> M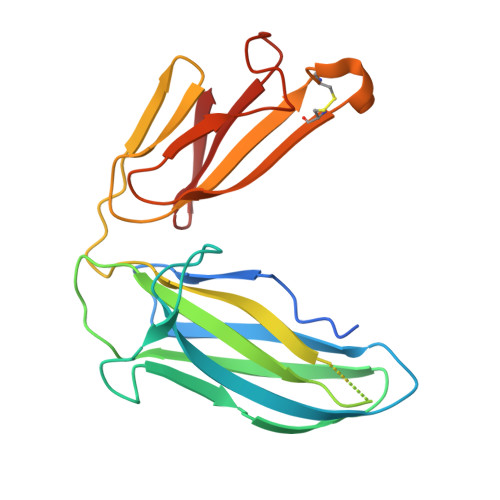AHHHHHHVDDDDKMLDVGDISSFMNSDSSTLSKTIQNSTDSGRLINIRLERLSSPLDDGQVIAMDKPDELLLTPASLLLPAQASEVIRFFYKGPADEKERYYRIVWFDQALSDAQRDNANRSAVATASARIGTILVVAPRQANYHFQYANGSLTNTGNATLRILAYGPCLKAANGKECKENYYLMPGKSRRFTRVDTADNKGRVALWQGDKFIPVK>LTCVKSNSIWFPTSEDCPDGQNLCFKRWQYISPRMYDFTRGCAATCPKPTNVRETIRCCGTDKCNK[2x]

The three-finger toxin (3FT) family is widely represented as structural motif, mainly in the Elapidae snake venoms, supporting various biological functions. This fold is characterized by three adjacent loops rich in β-pleated sheets emerging from a small globular core containing four invariant disulfide bridges. Despite high primary structure identity, often greater than 55%, muscarinic and adrenergic toxins exhibit distinct pharmacological profiles and clear functional differences. “Loop grafting” has been used to construct seven chimeric toxins to dissect how the affinity, selectivity and functionality for the muscarinic and adrenergic receptors depend on shuffling loops between various toxins.

Three chimeras were obtained by substituting loops of the MT7 toxin with the corresponding loop from the MT1. These chimeras were named MT7-1/1, MT7-1/2 and MT7-1/3, numbered for the respective grafted MT1 loop. The comparison of loop 3 from each of the two molecules in the asymmetric unit of MT7-1/3 compared to MT1 shows again an excellent match. The comparison of loop 2 from chain A of MT7-1/3 with loop 2 of MT1 shows that the replacement of loop 3 of MT7 for that of MT1 imposes a reorientation of the side chains to match that of MT1 although there is poor sequence identity. The situation with loop 3 is different because of the conserved interaction between loop 2 and the second strand of loop 3. To preserve the interaction we have observed that the side chain orientations on the top part of loop 2 tend to conform to those from the parent toxin. Indeed, in chimera MT7-1/3 the side chains on loop 2 execute a concerted rotation and adopt conformers that match closely those on MT1 loop 2. By least-squares fit we have an rmsd for MT1 vs MT7-1/3 of 2.87±0.08 Å while by SSM the value falls to an rmsd of 0.89 Å on 61 aligned residues with a 79% sequence identity. While loop 1 transfer has no significant effect on the toxin affinity for hM4, a moderate gain of function (5-fold) is observed with the grafting of loop 3. Notably, a two orders of magnitude increase in affinity for the α1A-adrenoceptor is achieved for chimeras MT7-1/1 and MT7-1/3 by the grafting of loop 1 or 3.>[2x]GSHMVPISFVFNRFPRMVRDLAKKMNKEVNFIMRGEDTELDRTF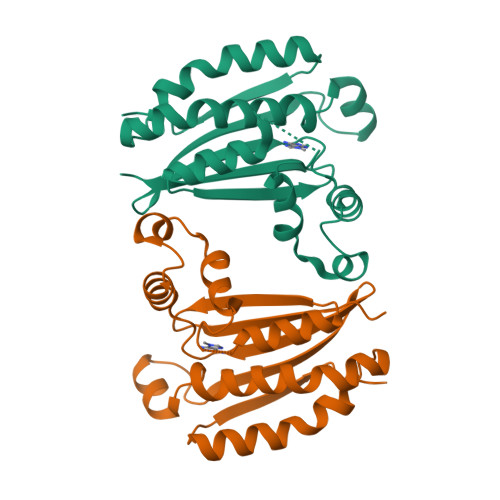VEEIGEPLLHLLRNAIDHGIEPKEERIAKGKPPIGTLILSARHEGNNVVIEVEDDGRGIDKEKIIRKAIEKGLIDESKAATLSDQEILNFLFVPGFSTKEKVSEVSGRGVGMDVVKNVVESLNGSISIESEKDKGTKVTIRLPLT>[2x]MYKEPFGVKVDFETGIIEGAKKSVRRLSDMEGYFVDERAWKELVEKEDPVV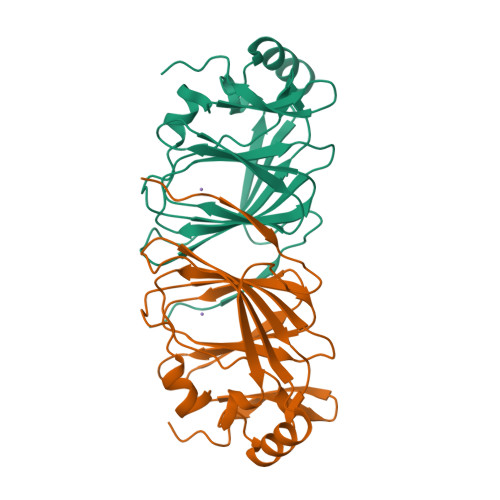YEVYAVEQEEKEGDLNFATTVLYPGKVGKEFFFTKGHFHAKLDRAEVYVALKGKGGMLLQTPEGDAKWISMEPGTVVYVPADWAHRTVNIGDEPFIFLAIYPADAGHDYGTIAEKGFSKIVIEENGEVKVVDNPRWKK(2S)-2-(3-{[AMINO(IMINO)METHYL]AMINO}PHENYL)-3-[(S)-HYDROXY(3-PHENYLPROPYL)PHOSPHORYL]PROPANOIC ACID 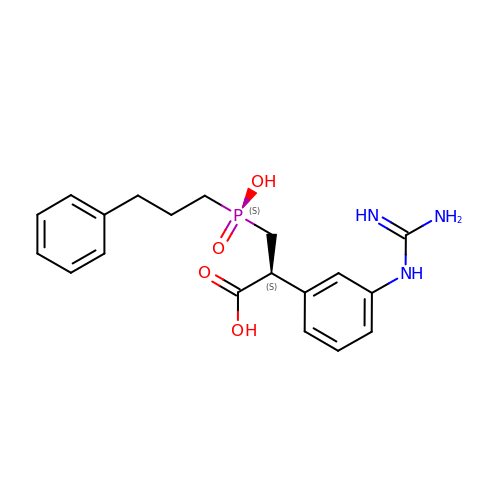| C19 H24 N3 O4 P | HFRHWTYCVGKGIE-KRWDZBQOSA-N>QGAVRKATAAEIAALPRQKVELVDPPFVHAHSQVAEGGPKVVEFTMVIEEKKIVIDDAGTEVHAMAFNGTVPGPLMVVHQDDYLELTLINPETNTLMHNIDFHAATGALGGGGLTEINPGEKTILRFKATKPGVFVYHCAPPGMVPWAVVSGMNGAIMVLPREGLHDGKGKALTYDKIYYVGEQDFYVPRDENGKYKKYEAPGDAYEDTVKVMRTLTPTHVVFNGAVGALTGDKAMTAAVGEKVLIVHSQANR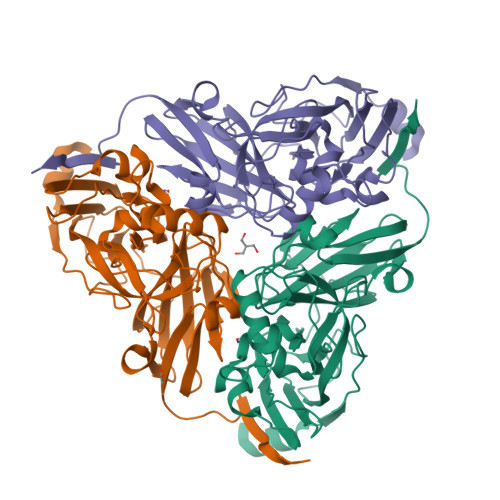DTRPHLIGGHGDYVWATGKFNTPPDVDQETWFIPGGAAGAAFYTFQQPGIYAYVNHNLIEAFELGAAAHFKVTGEWNDDLMTSVLAPSGT[3x]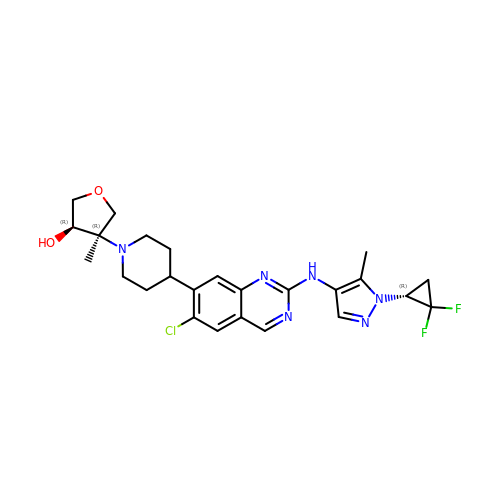(3R,4R)-4-{4-[6-chloro-2-({1-[(1R)-2,2-difluorocyclopropyl]-5-methyl-1H-pyrazol-4-yl}amino)quinazolin-7-yl]piperidin-1-yl}-4-methyloxolan-3-ol | C25 H29 Cl F2 N6 O2 | VFCYOTBJVABSBY-AOHZBQACSA-N>MHHHHHHGKPALEVLFQGPGSMRSLEDKNRTNTDDIRSLRVITAIKTPYLPDGRFDLQAYDDLVNTQIENGAEGVIVGGTTGEGQLMSWDEHIMLIGHTVNCFGGRIKVIGNTGSNSTREAIHATEQGFAMGMHGALHINPYYGKTSIEGMNAHFQTVLHMGPTIIYNVPGRTCQDIPPQVIFKLSQNPNMAGVKECVGNNRVEEYTEKGIVVWSGNDDQCHDSRWDHGAT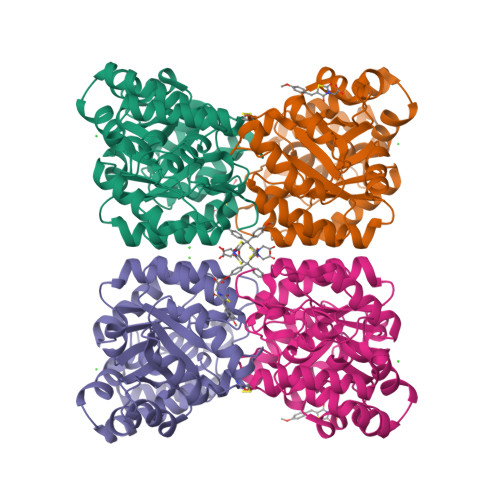GVISVTSNLVPGLMRKLMFEGRNSALNAKLLPLMDWLFQEPNPIGVNTALAQLGVARPVFRLPYVPLPLSKRIEFVKLVKEIGREHFVGDRDVQVLDDDDFILIGRY[2x]>MTDKLTSLRQYTTVVADTGDIAAMKLYQPQDATTNPSLILNAAQIPEYRKLIDDAVAWAKQQSNDRAQQIVDATDKLAVNIGLEILKLVPGRISTEVDARLSYDTEASIAKAKRLIKLYNDAGISNDRILIKLASTWQGIRAAEQLEKEGINCNLTLLFSFAQARACAEAGVFLISPFVGRILDWYKANTDKKEYAPAEDPGVVSVSEIYQYYKEHGYETVVMGAS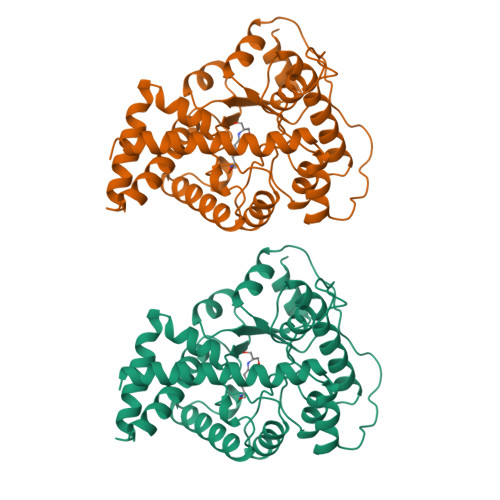FRNIGEILELAGCDRLTIAPALLKELAESEGAIERKLSYTGEVKARPARITESEFLWQHNQDPMAVDKLAEGIRKFAIDQEKLEKMIGDLL[2x]Interestingly, Connolly and colleagues found that archaeal B‐family DNA polymerases have evolved a so called “read ahead” mechanism to sense uracil in the template strand, stalling DNA polymerase promoted DNA synthesis of nascent DNA before the deaminated nucleobase reaches the polymerase active site. Here we report on three new crystal structures of the archaeal B‐family DNA polymerase from Thermococcus kodakarensis (KOD) DNA polymerase in complex with primer and template strands that have extended single stranded DNA template 5’‐overhangs. These overhangs contain either the canonical nucleobases as well as uracil or hypoxanthine, respectively, and provide unprecedented structural insights into their recognition by archaeal B‐family DNA polymerases. The template overhang binds into a positively charged crevice between the N‐terminal and the exonuclease domain of the DNA polymerase.

[4f] To study this in our context we performed analogous crystallization experiments with a hypoxanthine‐containing 21 nt template. The experiments resulted in a binary complex with the p/t complex bound by the enzyme in an open state, characterized by an open finger domain and no substrate triphosphate bound. All single stranded nucleotides could be modelled, however, the single stranded nucleotides C+2, A+3 and A+4 show weaker electron density and hence more flexibility compared to the rest of the template and compared to the same positions in KOD‐U. These nucleotides may adopt different alternate conformations. The first single stranded nucleotide T+1 does not stack on the p/t duplex but is rotated to the side and the nucleobase is twisted by nearly 90° compared to the p/t duplex end. Again the backbone amide nitrogen atoms of Tyr37 and Ile114 interact with the exocyclic O6 and the ring N3 of hypoxanthine, respectively while a water molecule, that is bridged by hydrogen bonds to Glu111, Tyr37 and Arg119 interacts with the 1‐NH group. The B‐factors of hypoxanthine are lower compared to the neighboring nucleotides which speaks for a stabilization in the binding pocket. Superimposition of guanine on hypoxanthine reveals a clash of 2‐NH2 with the main chain oxygen of Glu111 (nearest distance around 2.2 Å) or the side chain of Ile114 (nearest distance around 2.7 Å) explaining guanine exclusion. The only significant difference is a water molecule which participates in hydrogen bonds to 3‐NH of uracil and 1‐NH of hypoxanthine. In KOD‐H, the water molecule is displaced by 0.9 Å to accommodate the bigger nucleobase.

> MILDTDYITEDGKPVIRIFKKENGEFKIEYDRTFEPYFYALLKDDSAIEEVKKITAERHGTVVTVKRVEKVQKKFLGRPVEVWKLYFTHPQDVPAIRDKIREHPAVIDIYEYDIPFAKRYLIDKGLVPMEGDEELKMLAFAIATLYHEGEEFAEGPILMISYADEEGARVITWKNVDLPYVDVVSTEREMIKRFLRVVKEKDPDVLITYNGDNFDFAYLKKRCEKLGINFALGRDGSEPKIQRMGDRFAVEVKGRIHFDLYPVIRRTINLPTYTLEAVYEAVFGQPKEKVYAEEITTAWETGENLERVARYSMEDAKVTYELGKEFLPMEAQLSRLIGQSLWDVSRSSTGNLVEWFLLRKAYERNELAPNKPDEKELARRRQSYEGGYVKEPERGLWENIVYLDFRSLYPSIIITHNVSPDTLNREGCKEYDVAPQVGHRFCKDFPGFIPSLLGDLLEERQKIKKKMKATIDPIERKLLDYRQRAIKILANSYYGYYGYARARWYCKECAESVTAWGREYITMTIKEIEEKYGFKVIYSDTDGFFATIPGADAETVKKKAMEFLKYINAKLPGALELEYEGFYKRGFFVTKKKYAVIDEEGKITTRGLEIVRRDWSEIAKETQARVLEALLKDGDVEKAVRIVKEVTEKLSKYEVPPEKLVIHEQITRDLKDYKATGPHVAVAKRLAARGVKIRPGTVISYIVLKGSGRIGDRAIPFDEFDPTKHKYDAEYYIENQVLPAVERILRAFGYRKEDLRYQKTRQVGLSAWLKPKGT Clostridial collagenases are among the most efficient enzymes to degrade by far the most predominant protein in the biosphere. Clostridia employ collagenases for nutrition (e.g. saprophytic strains) and host colonization (1–3). They are large multidomain proteins of ∼115 kDa belonging to the gluzincin superfamily of metalloproteases. Here we present the crystal structures of the peptidase domains of ColH and ColT and the collagenase unit of ColG in the presence and absence of the peptidic inhibitor isoamylphosphonyl-Gly-Pro-Ala bound to the active site.

Although the previously reported ColG crystals contained the PKD-like domain in addition to the collagenase unit, the PKD-like domain remained largely disordered. This disorder is presumably related to the presence of citrate in the crystallization buffer, which titrates away Ca2+ ions. Because the crystal packing did not tolerate rebuffering to introduce calcium, we produced and crystallized an isolated PKD-like domain spanning residues Asn795–Asn880 to investigate its calcium-binding properties. To verify the proposed calcium binding site in the PKD-like domain, the crystal structure of an N-terminally extended construct of the PKD-like domain of ColG (Asn795–Asn880) was determined in the presence of 10 mm calcium at 0.99 Å resolution. In this orthorhombic crystal form, we identified six proteinaceous ligands, namely Asn795, Lys796, Asp825, Asp864, and both of the carboxylate oxygens of Asp823, which together with a seventh water ligand coordinate the calcium ion in a pentagonal-bipyramidal geometry. In addition, an N-terminally further extended PKD construct (Ile792–Asn880) was crystallized in the same conditions as the Asn795–Asn880, but the additional residues (Ile792, Ser793, and Asn794) could not be traced in the electron density, indicating their flexibility even in the presence of calcium (data not shown). Notably, in both PKD variants (Ile792–Asn880 and Asn795–Asn880), the calcium could not be extracted by incubating the respective crystals for up to 4 h with 100 mm EDTA.

> GGTISNNKAPIAKVTGPSTGAVGRNIEFSGKDSKDEDGKIVSYDWDFGDGATSRGKNSVHAYKKAGTYNVTLKVTDDKGATATESFTIEIKN>SNAKNASVITVGNEILKGRTVNTNAAFIGNFLTYHGYQVRRGFVVMDDLDEIGWAFRVALEVSDLVVSSGGLGPTFDDMTVEGFAKCIGQDLRIDEDALAMIKKKYGQADLTPQRLKMAKIPPSCRPIENPVGTAPGLICAVGG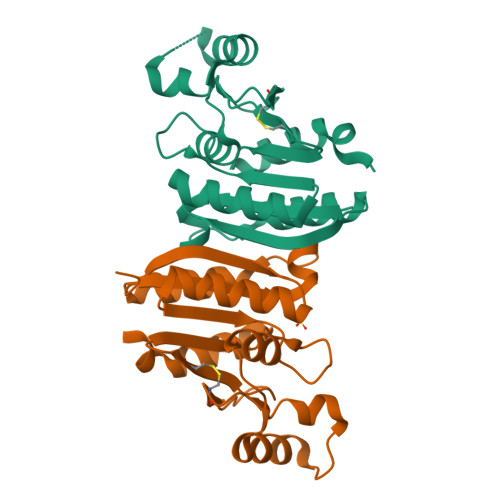KKVIILPGVPKEMEALLKAMEKDIIIPD[2x]> AMTYHLDVVSAEQQMFSGLVEKIQVTGSEGELGIYPGHAPLLTAIKPGMIRIVKQHGHEEFIYLSGGILEVQPGNVTVLADTAIRGQDLDEARAMEAKRKAEEHISSSHGDVDYAQASAELAKAIAQLRVIELTKKAM;> KITKAMEMVAASKMRKSQDRMAASRPYAETMRKVIGHLAHGNLEYKHPYLEDRDVKRVGYLVVSTDRGLCGGLNINLFKKLLAEMKTWTDKGVQCDLAMIGSKGVSFFNSVGGNVVAQVTGMGDNPSLSELIGPVKVMLQAYDEGRLDKLYIVSNKFINTMSQVPTISQLLPLPASDDDDLKHKSWDYLYEPDPK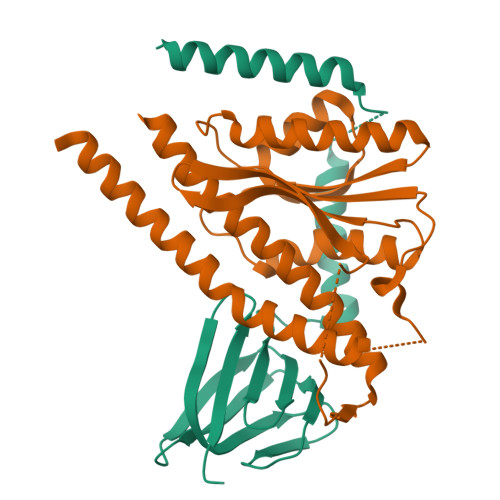ALLDTLLRRYVESQVYQGVVENLASEQAARMVAMK>MRKLNPALEFRDFIQVLKDEDDLIEITEEIDPNLEVGAIMRKAYESHLPAPLFKNLKGASKDLFSILGCPAGLRSKEKGDHGRIAHHLGLDPKTTIKEIIDYLLECKEKEPLPPITVPVSSAPCKTHILSEEKIHLQSLPTPYLHVSDGGKYLQTYGMWILQTPDKKWTNWSIARGMVVDDKHITGLVIKPQHIRQIADSWAAIGKANEIPFALCFGVPPAAILVSSMPIPEGVSESDYVGAILGESVPVVKCETNDLMVPATSEMVFEGTLSLTDTHLEGPFGEMHGYVFKSQGHPCPLYTVKAMSYRDNAILPVSNPGLCTDETHTLIGSLVATEAKELAIESGLPILDAFMPYEAQALWLILKVDLKGLQALKTTPEEFCKKVGDIYFRTKVGFIVHEIILVADDIDIFNFKEVIWAYVTRHTPVADQMAFDDVTSFPLAPFVSQSSRSKTMKGGKCVTNCIFRQQYERSFDYITCNFEKGYPKGLVDKVNENWKRY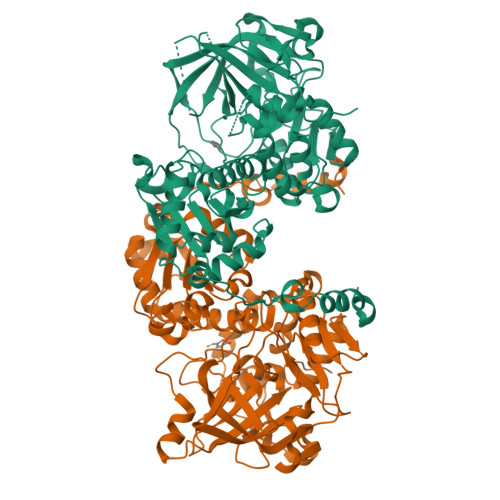GYK[8x]Calcium homeostasis modulator 1 (CALHM1) is a voltage-dependent channel involved in neuromodulation and gustatory signaling. CALHM1 is the recently identified member of a large-pore channel that permeates ions, including Ca2+, Na+, K+, and Cl−, and small molecules, such as ATP, in a voltage-dependent manner. Furthermore, the ATP efflux through the CALHM1 channel in type II gustatory cells and the subsequent purinergic signaling has been shown to facilitate the perception of sweet, bitter, and umami taste sensations. Our studies here showed that the human and chicken CALHM1s have a conserved structural fold, oligomeric assembly pattern, and a phospholipid-filled hydrophobic pocket for controlling channel functions.

To compare structures and assembly patterns of mammalian and non-mammalian CALHM1 channels, we determined the cryo-EM structure of human CALHM1, as well as that of chicken CALHM1 prepared using an identical protocol. Our single-particle cryoEM resulted in the octameric chCALHM1Δct and hCALHM1Δct structures, resolved at the overall resolutions of 3.36 and 3.76 Å, respectively. The overall protomer organization is similar between chCALHM1Δct and hCALHM1Δct (RMSD = 1.016 Å over 186 Cα positions), illustrating the structural conservation despite differences in amino acid sequences (72% identity and 90.6% similarity within CALHM1Δct). The structures of chCALHM1Δct and hCALHM1Δct are most similar within the TMD regions (RMSD = 0.826 Å; over 140 Cα positions), whereas that of CTH is more variable (RMSD = 1.294 Å; over 49 Cα positions). In our hCALHM1Δct structure, the cryo-EM density was resolved up to Pro85 but not Pro86. However, our chCALHM1Δct map allowed the modeling of residues 85-90 and revealed that these residues are located outside the center pore, indicating that Pro86 is likely not directly involved in the alteration of channel functions. In fact, many of the subunit interface residues at TMD2, TMD4, and CTH are conserved among human, mouse, chicken, killifish, and zebrafish orthologues (*). It is worth mentioning that we observed octameric and nonameric assembly as assessed by the ‘top’ views of 2D classification in both chCALHM1Δct and hCALHM1Δct; however, we could only 3D reconstruct the octameric channel as the majority of the particles belong to the octameric species. In contrast, the full-length chCALHM1 that was trypsinized post-purification displayed only octameric architectures. Inspection of the hCALHM1Δct and chCALHM1Δct structures reveals a hydrophobic pocket ~15 Å in length (parallel to the TMDs) and 10 Å wide, located between TMD3 and TMD4 of one subunit and TMD2 of the neighboring subunit. In both hCALHM1Δct and chCALHM1Δct, we observe phospholipid-like density nestled into this pocket, which appears to fortify the local architecture by interacting with the hydrophobic residues in the pocket.

>[8x]MDKFRMVFQFLQSNQESFMSGICGIMALASAQLYSAFDFNCPCLPRYNLAYGLGVLLVPPLILFLLGFVLNNNVSMLAEEWRRPQGQRQKDAAVLRYMFCSMVQRAMIAPAVWVSVTLLDGKCITCAFCTSLPVEALGNASHHGLPQGEVKRVLARIPCKEIYDGQELIANEVAVRYLRCISQALGWCFVLLMTTLAFLVRSLRPCFTQAVFLKSRYWSHYIDIERKLFDETCAEHAKSFAKVCIQQFFQGMSKDLTATHCHPPRKAPTDAGEASEKLLGITDWDTMNIALGSAWSHPQFEK> GGUUGCCGAA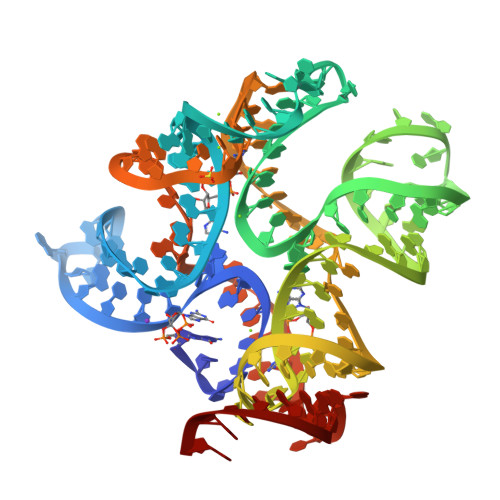UCCAUAUGUGGUACGGAGGAACCGCUUUUUGGGGUUAAUCUGCAGUGAAGCUGCAGUAGGGAUACCUUCUGUCCCGCACCCGACAGCUAACUCCGGAGGCAAUAAAGGAAGGAG> GSHMSGIALSRLAQERKAWRKDHPFGFVAVPTKNPDGTMNLMNWECAIPGKKGTPWEGGLFKLRMLFKDDYPSSPPKCKFEPPLFHPNVYPSGTVCLSILEEDKDWRPAITIKQILLGIQELLNEPNIQA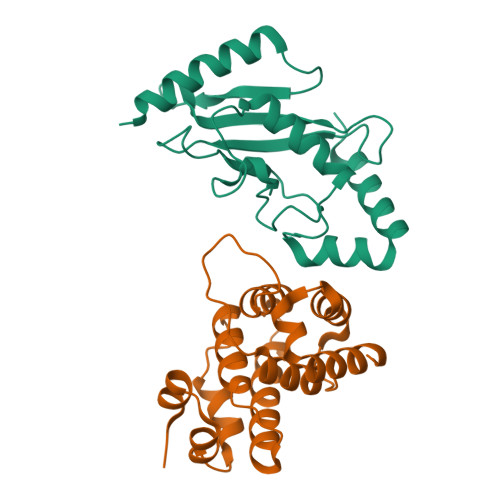PAQAEAYTIYCQNRVEYEKRVRAQAKKFAPS;> STGEPAPVLSSPPPADVSTFLAFPSPEKLLRLGPKSSVLIAQQTDTSDPEKVVSAFLKVSSVFKDEATVRMAVQDAVDALMQKAFNSSSFNSNTFLTRLLVHMGLLKSEDKVKAIANLYGPLMALNHMVQQDYFPKALAPLLLAFVTKPNSALESCSFARHSLLQTLYKV(4S)-6-CHLORO-3-{2-[4-(FURAN-2-YLCARBONYL)PIPERAZIN-1-YL]ETHYL}-2-METHYL-4-PHENYL-3,4-DIHYDROQUINAZOLINE | C26 H27 Cl N4 O2 | 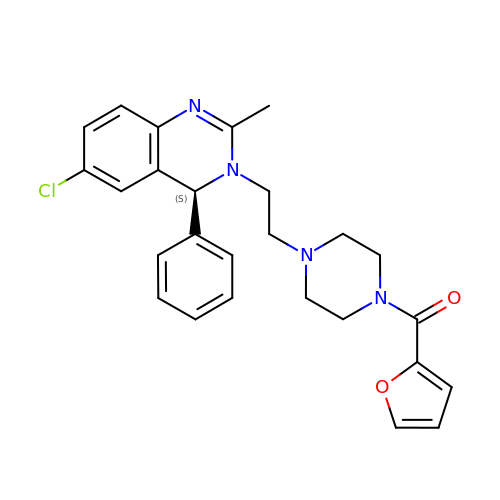LZBVDXKZVXPKHV-VWLOTQADSA-N>MTVLIVTFSRDNESIPLVIKAIEAMGKKAFRFDTDRFPTEVKVDLYSGGQKGGIITDGDQKLELKEVSAVWYRRMRYGLKLPDGMDSQFREASLKECRLSIRGMIASLSGFHLDPIAKVDHANHKQLQLQVARQLGLLIPGTLTSNNPEAVKQFAQEFEATGIVTKMLSQFAIYGDKQEEMVVFTSPVTKEDLDNLEGLQFCPMTFQENIPKALELRITIVGEQIFTAAINSQQLDGAIYDWRKEGRALHQQWQPYDLPKTIEKQLLELMKYFGLNYGAIDMIVTPDERYIFLEINPVGEFFWLELYPPYFPISQAIAEILVN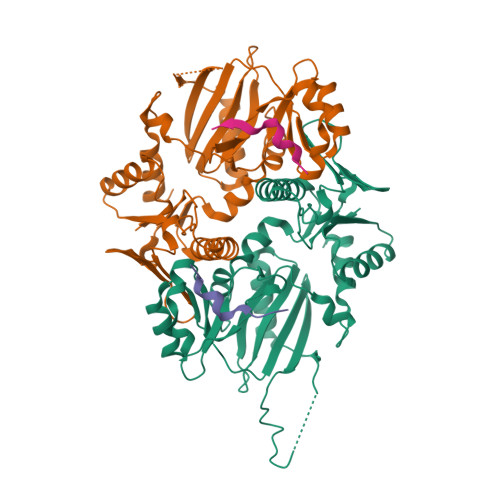SAAAHHHHHH[8x];>[8x]MAYPNDQQGKALPFFARFLSVSKEESSIKSPSPDHEISTRKYPSDWEEW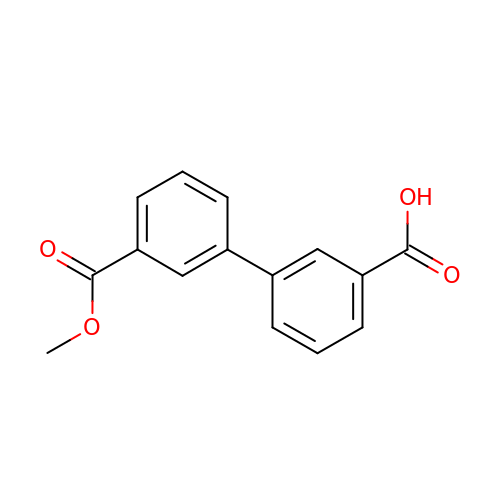3-(3-methoxycarbonylphenyl)benzoic acid | C15 H12 O4 | CJWQBLCGSMIQJV-UHFFFAOYSA-N>[2x]MKFAEHLSAHITPEWRKQYIQYEAFKDMLYSAQDQAPSVEVTDEDTVKRYFAKFEEKFFQTCEKELAKINTFYSEKLAEAQRRFATLQNELQSSLDAQKESTGVTTLRQRRKPVFHLSHEERVQHRNIKDLKLAFSEFYLSLILLQNYQNLNFTGFRKILKKHDKILETSRGADWRVAHVEVAPFYTCKKINQLISETEAVVTNELEDGDRQKAMKRLRVPPLGAAQPAPAWTTFRVGLFCGIFIVLNITLVLAAVFKLETDRSIWPLIRIYRGGFLLIEFLFLLGINTYGWRQAGVNHVLIFELNPRSNLSHQHLFEIAGFLGILWCLSLLACFFAPISVIPTYVYPLALYGFMVFFLINPTKTFYYKSRFWLLKLLFRVFTAPFHKVGFADFWLADQLNSLSVILMDLEYMICFYSLELKWD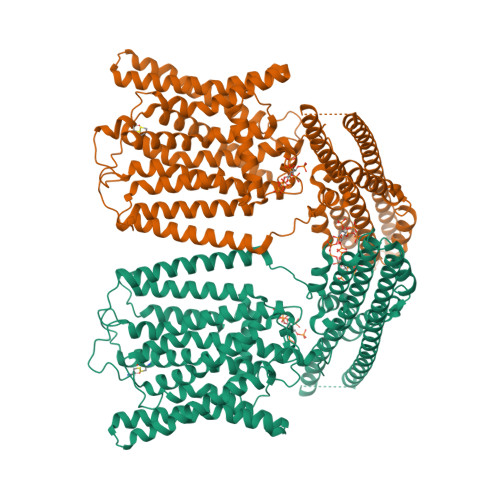ESKGLLPNNSEESGICHKYTYGVRAIVQCIPAWLRFIQCLRRYRDTKRAFPHLVNAGKYSTTFFMVTFAALYSTHKERGHSDTMVFFYLWIVFYIISSCYTLIWDLKMDWGLFDKNAGENTFLREEIVYPQKAYYYCAIIEDVILRFAWTIQISITSTTLLPHSGDIIATVFAPLEVFRRFVWNFFRLENEHLNNCGEFRAVRDISV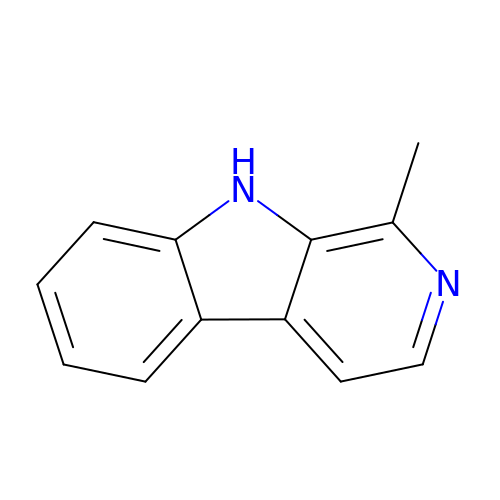1-methyl-9H-pyrido[3,4-b]indole | C12 H10 N2 | PSFDQSOCUJVVGF-UHFFFAOYSA-N> DTGPTGIKYDLDRHQYNYVDAVCYENRLHWFAKYFPYLVLLHTLIFLACSNFWFKFPRTSSKLEHFVSILLKCFDSPWTTRALSETVVEESDPKPAFSKMNGSMDKKSSTVSEDVEATVPMLQRTKSRIEQGIVDRSETGVLDKKEGEQAKALFEKVKKFRTHVEEGDIVYRLYMRQTIIKVIKFALIICYTVYYVHNIKFDVDCTVDIESLTGYRTYRCAHPLATLFKILASFYISLVIFYGLICMYTLWWMLRRSLKKYSFESIREESSYSDIPDVKNDFAFMLHLIDQYDPLYSKRFAVFLSEVSENKLRQLNLNNEWTLDKLRQRLTKNAQDKLELHLFMLSGIPDTVFDLVELEVLKLELIPDVTIPPSIAQLTGLKELWLYHTAAKIEAPALAFLRENLRALHIKFTDIKEIPLWIYSLKTLEELHLTG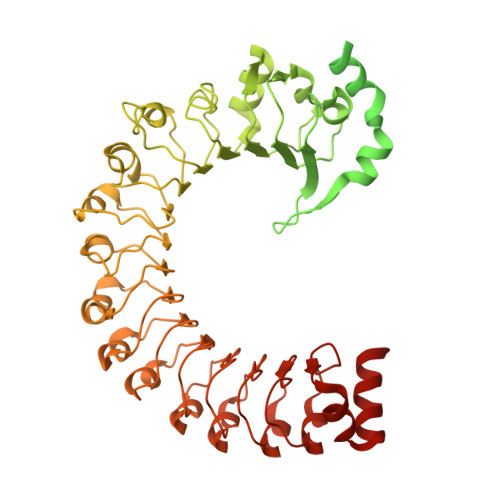NLSAENNRYIVIDGLRELKRLKVLRLKSNLSKLPQVVTDVGVHLQKLSINNEGTKLIVLNSLKKMVNLTELELIRCDLERIPHSIFSLHNLQEIDLKDNNLKTIEEIISFQHLHRLTCLKLWYNHIAYIPIQIGNLTNLERLYLNRNKIEKIPTQLFYCRKLRYLDLSHNNLTFLPADIGLLQNLQNLAVTANRIEALPPELFQCRKLRALHLGNNVLQSLPSRVGELTNLTQIELRGNRLECLPVELGECPLLKRSGLVVEEDLFSTLPPEVKERLWRADKEQASNSLEVLFQ>MSNSVKSPSDHVGDVGRRNYPMSARTLVTQEQVWAATAKCAKKIAADYKDFHLTADNPLYLLCVLKGSFIFTADLARFLADEGVPVKVEFICASSYGSGVETSGQVRMLLDVRDSVENRHIMLVEDIVDSAIT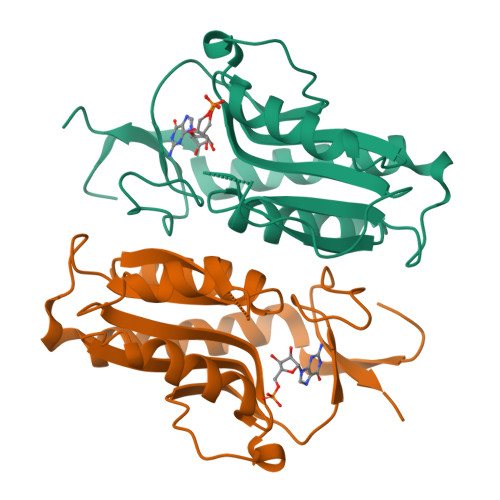LQYLMRFMLAKKPASLKTVVLLDKPSGRKVDVLVDYPVITIPRAFVIGYGMDFAESYRELRDICVLKKEYYEKAESKL[2x]Streptococcus mutans, a known etiological agent in the pathogenesis of dental caries, expresses three genetically distinct types of glucosyltransferases (Gtfs; also known as glucansucrases): GtfB (GTF-I), GtfC (GTF-SI) and GtfD (GTF-S). GtfC synthesizes both soluble and insoluble glucans (α-1,3 and α-1,6 glycosidic linkages), while GtfB and GtfD only synthesize insoluble glucans (mostly α-1,3 linkages) and soluble glucans (mostly α-1,6 linkages), respectively. All three enzymes belong to glycoside hydrolase family 70 (GH70), which cleaves the glycosidic bond between the glucose and fructose moieties in sucrose during catalysis. While fructose is released, the enzymatically produced glucose molecules are sequentially fused into a growing glucan chain and, depending on whether a 1,3- or 1,6-linkage is formed, the resultant product is either an insoluble or a soluble glucan, respectively.

More importantly, we have now co-crystallized the GtfB with acarbose, which highlights differences in the interactions with ligands in these distinct Gtfs. With this work, apo structures and inhibitor-complex structures with acarbose are now available for the catalytic domains of GtfC and GtfB. The four rings of acarbose occupy subsites −1, +1, +2 and +3. However, using a hydrogen-bond distance cutoff of 3.2 Å, 12 hydrogen bonds were observed in GtfB-CD, while eight hydrogen bonds were observed in GtfC-CD. A surface diagram colored by electrostatic potential shows that the active-site pocket is small and negatively charged. An acceptor molecule or part of a growing glucan chain has to bind farther out in subsites +2 and +3, as indicated by acarbose binding, or beyond. In conclusion, our work demonstrates that GtfB-CD is quite similar to GtfC-CD, although their adherence to acarbose differs significantly.

>[8x]LHFDETGAYTDTSIDTVNKDIVTTRSNLYKKYNQVYDRSAQSFEHVDHYLTAESWYRPKYILKDGKTWTQSTEKDFRPLLMTWWPSQETQRQYVNYMNAQLGINKTYDDTSNQLQLNIAAATIQAKIEAKITTLKNTDWLRQTISAFVKTQSAWNSDSEKPFDDHLQNGAVLYDNEGKLTPYANSNYRILNRTPTNQTGKKDPRYTADNTIGGYEFLLANDVDNSNPVVQAEQLNWLHFLMNFGNIYANDPDANFDSIRVDAVDNVDADLLQIAGDYLKAAKGIHKNDKAANDHLSILEAWSDNDTPYLHDDGDNMINMDNKLRLSLLFSLAKPLNQRSGMNPLITNSLVNRTDDNAETAAVPSYSFIRAHDSEVQDLIRDIIKAEINPNVVGYSFTMEEIKKAFEIYNKDLLATEKKYTHYNTALSYALLLTNKSSVPRVYYGDMFTDDGQYMAHKTINYEAIETLLKARIKYVSGGQAMRNQQVGNSEIITSVRYGKGALKATDTGDRTTRTSGVAVIEGNNPSLRLKASDRVVVNMGAAHKNQAYRPLLLTTDNGIKAYHSDQEAAGLVRYTNDRGELIFTAADIKGYANPQVSGYLGVWVPVGAAADQDVRVAASTAPSTDGKSVHQNAALDSRVMFEGFSNFQAFATKKEEYTNVVIAKNVDKFAEWGVTDFEMAPQYVSSTDGSFLDSVIQNGYAFTDRYDLGISKPNKYGTADDLVKAIKALHSKGIKVMADWVPDQMYAFPEKEVVTATRVDKFGKPVEGSQIKSVLYVADSKSSGKDQQAKYGGAFLEELQAKYPELFARKQISTGVPMDPSVKIKQWSAKYFNGTNILGRGAGYVLKDQATNTYFNISDNKLEHHHHHH2-{[(2,5-DICHLOROPHENYL)METHYL]SULFANYL}-5-ETHYL-[1,2,4]TRIAZOLO[1,5-A]PYRIMIDIN-7-OL 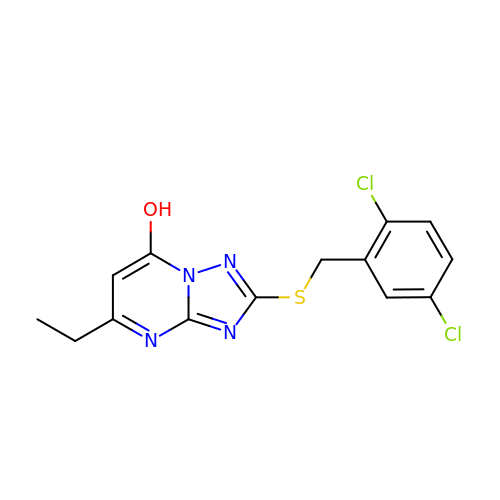| C14 H12 Cl2 N4 O S | HVAYQTZQQDSNCH-UHFFFAOYSA-N> MGRMLTIRVFKYDPQSAVSKPHFQEYKIEEAPSMTIFIVLNMIRETYDPDLNFDFVCRAGICGSCGMMINGRPSLACRTLTKDFEDGVITLLPLPAFKLIKDLSVDTGNWFNGMSQRVESWIHAQKEHDISKLEERIEPEVAQEVFELDRCIECGCC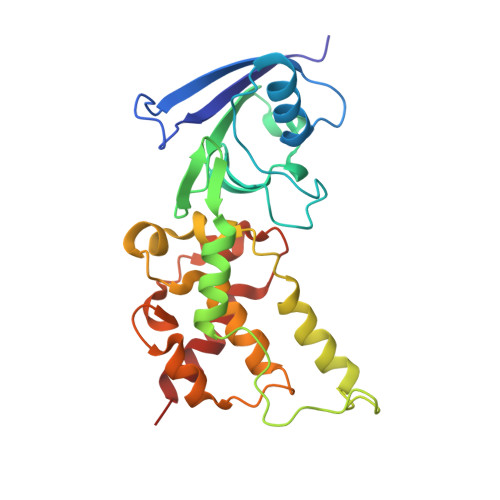IAACGTKIMREDFVGAAGLNRVVRFMIDPHDERTDEDYYELIGDDDGVFGCMTLLACHDVCPKNLPLQSKIAYLRRKMVSVN> SKLIHVPKEDNSKEVTLDSLLEEGVLDKEIHKA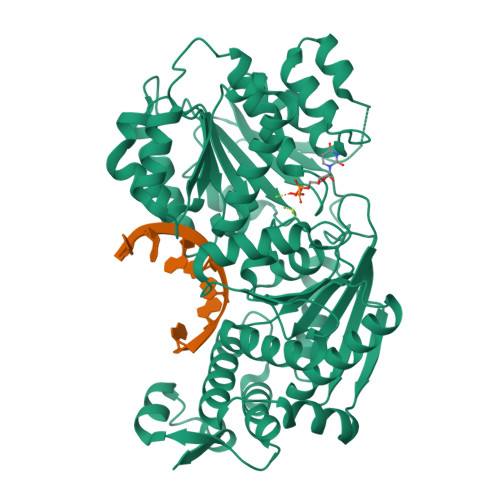ITRMEFPGLTPVQQKTIKPILSSEDHDVIARAKTGTGKTFAFLIPIFQHLINTKFDSQYMVKAVIVAPTRDLALQIEAEVKKIHDMNYGLKKYACVSLVGGTDFRAAMNKMNKLRPNIVIATPGRLIDVLEKYSNKFFRFVDYKVLDEADRLLEIGFRDDLETISGILNEKNSKSADNIKTLLFSATLDDKVQKLANNIMNKKECLFLDTVDKNEPEAHERIDQSVVISEKFANSIFAAVEHIKKQIKERDSNYKAIIFAPTVKFTSFLCSILKNEFKKDLPILEFHGKITQNKRTSLVKRFKKDESGILVCTDVGARGMDFPNVHEVLQIGVPSELANYIHRIGRTARSGKEGSSVLFICKDELPFVRELEDAKNIVIAKQEKYEPSEEIKSEVLEAVTEEPEDISDIVISLISSYRSCIKEYRFSERRILPEIASTYGVLLNDPQLKIPVSRRFLDKLGLSRSPIGKAMFEIRD>[7x]MALSDLQVFNDWAYKTMSEVLDQQVELFNGATRGAIILRSAGNTGDLSEAAFWAKIQGLVRPRDPYSNADVAAKDLRQLVDNTIKVASGTPPINIPPSMLRWIQKNPQEAGAVIGQQLAGDTMQDMLNNGLAAGKAAFTAGGAVHDISAA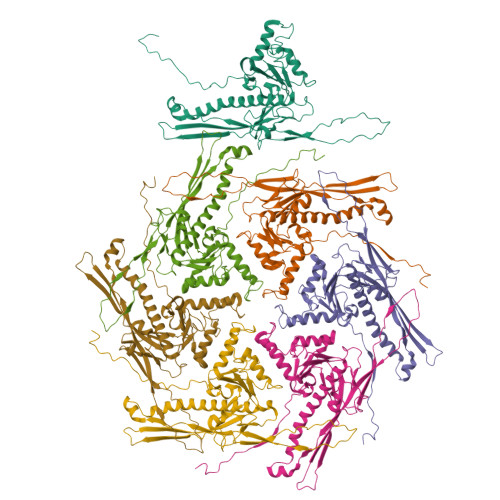GTGLMTQRAFNAAQRIFGDRSTDIQVWVSHSSPLFDLYDNALANAEQLYVFGTVNVRADAFGRPIIITDSPALVSGAAETLRHSTLGLTTGAILIEQNQDFDSTVVDGTGKQNITRQYQAEWSYNLGVNGYAYDIATGGKAPNPTALATAANWDKISTSIKDTGGVVLVTK> S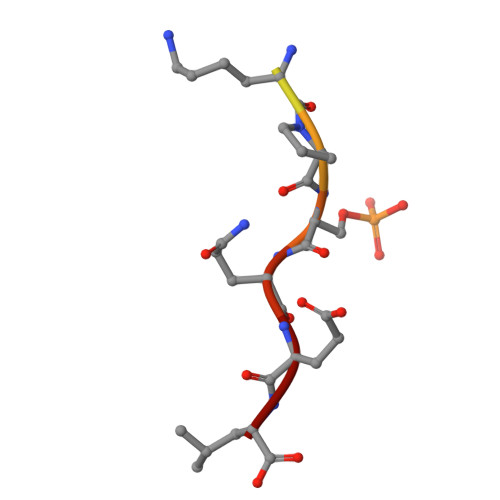GRTGKPSQEL> X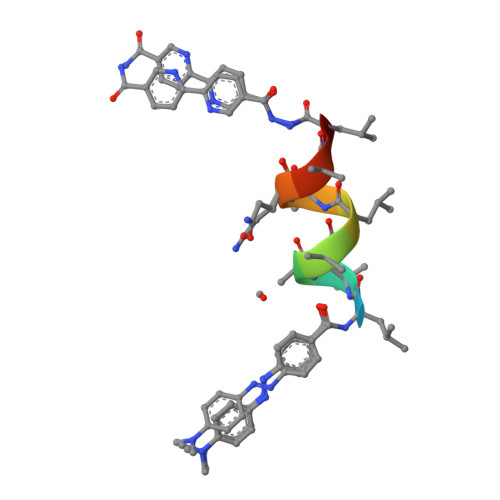LAAALAQALX>[2x]MIKI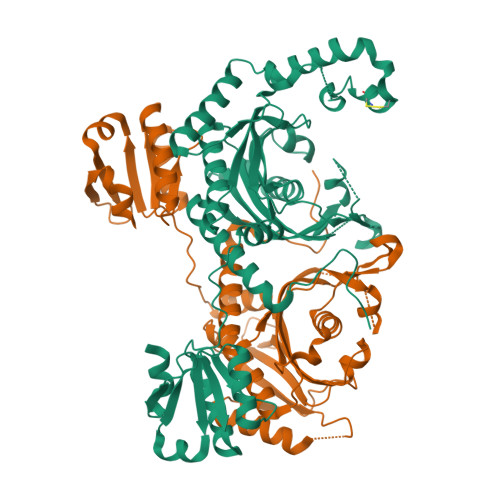PRGTQDILPEDSKKWRYIENQLDELMTFYNYKEIRTPIFESTDLFARGVGDSTDVVQKEMYTFKDKGDRSITLRPEGTAAVVRSYIEHKMQGNPNQPIKLYYNGPMFRYERKQKGRYRQFNQFGVEAIGAENPSVDAEVLAMVMHIYQSFGLKHLKLVINSVGDMASRKEYNEALVKHFEPVIHEFCSDCQSRLHTDPMRILDCKVDRDKEAIKTAPRITDFLNEESKAYYEQVKAYLDDLGIPYTEDPNLVRGLDYYTHTAFELMMDNPNYDGAITTLCGGGRYNGLLELLDGPSETGIGFALSIERLLLALEEEGIELDIEENLDLFIVTMGDQADRYAVKLLNHLRHNGIKADKDYLQRKIKGQMKQADRLGAKFTIVIGDQELENNKIDVKNMTTGESETIELDALVEYFKK>[2x]LKFSPQLLSLLSLKTSLSGPPSAFQDWKVPVNGQNDAVWCSWSGVVCDNVTAQVISLDLSHRNLSGRIPIQIRYLSSLLYLNL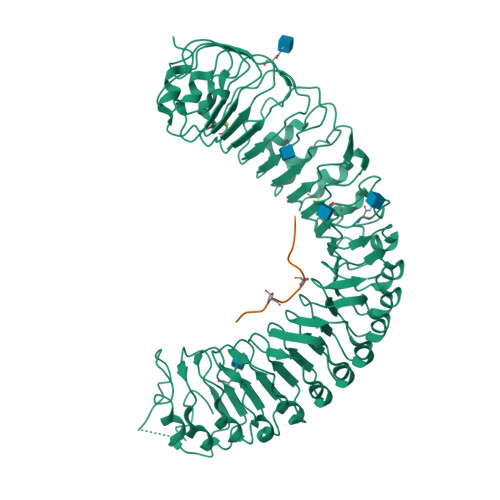SGNSLEGSFPTSIFDLTKLTTLDISRNSFDSSFPPGISKLKFLKVFNAFSNNFEGLLPSDVSRLRFLEELNFGGSYFEGEIPAAYGGLQRLKFIHLAGNVLGGKLPPRLGLLTELQHMEIGYNHFNGNIPSEFALLSNLKYFDVSNCSLSGSLPQELGNLSNLETLFLFQNGFTGEIPESYSNLKSLKLLDFSSNQLSGSIPSGFSTLKNLTWLSLISNNLSGEVPEGIGELPELTTLFLWNNNFTGVLPHKLGSNGKLETMDVSNNSFTGTIPSSLCHGNKLYKLILFSNMFEGELPKSLTRCESLWRFRSQNNRLNGTIPIGFGSLRNLTFVDLSNNRFTDQIPADFATAPVLQYLNLSTNFFHRKLPENIWKAPNLQIFSASFSNLIGEIPNYVGCKSFYRIELQGNSLNGTIPWDIGHCEKLLCLNLSQNHLNGIIPWEISTLPSIADVDLSHNLLTGTIPSDFGSSKTITTFNVSYNQLIGPIPSGSFAHLNPSFFSSNEGLCGDLVGKPCNSDRFNAGNADIDG;>[2x]HEVPSGPNPISN> GRREQTHRAVFRFIPRHPDELELDVDDPVLVEA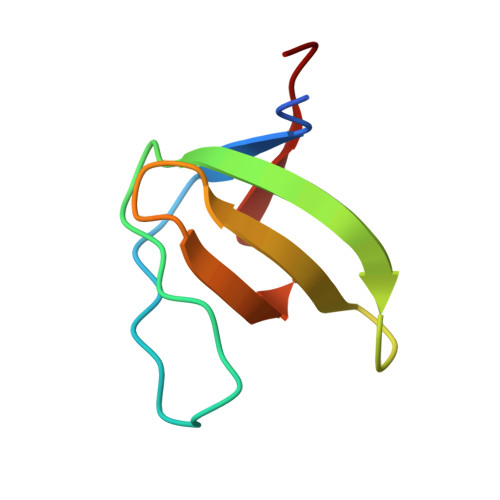EEDDFWFRGFNMRTGERGVFPAFYAHAVPG> MAEQVKPAGVKPKGTVPPPKGNAPAPKANGAPGGASVIKEQDAAKMRRFLFQRTETRSTKWYQIFDTEKLDDEQVVGGHLALLGVLGFIMGIYYISGIQVFPWGAPGFHDNWFYLTIKPRMVSLGIDTYSTKTADLEAAGARLLGWAAFHFLVGSVLIFGGWRHWTHNLTNPFTGRCGNFRDFRFLGKFGDVVFNGTSAKSYKEALGPHAVYMSLLFLGWGIVMWAILGFAPIPDFQTINSETFMSFVFAVIFFALGIYWWNNPPNAAIHLNDDMKAAFSVHLTAIGYINIALGCIAFVAFQQPSFAPYYKELDKLVFYLYGEPFNRVSFNFVEQGGKVISGAKEFADFPAYAILPKSGEAFGMARVVTNLIVFNHIICGVLYVFAGVYHGGQYLLKIQLNGMYNQIKSIWITKGRDQEVQVKILGTVMALCFATMLSVYAVIVWNTICELNIFGTNITMSFYWLKPLPIFQWMFADPSINDWVMAHVITAGSLFSLIALVRIAFFAHTSPLWDDLGLKKNSYSFPCLGPVYGGTCGVSIQDQLWFAMLWGIKGLSAVCWYIDGAWIASMMYGVPAADAKAWDSIAHLHHHYTSGIFYYF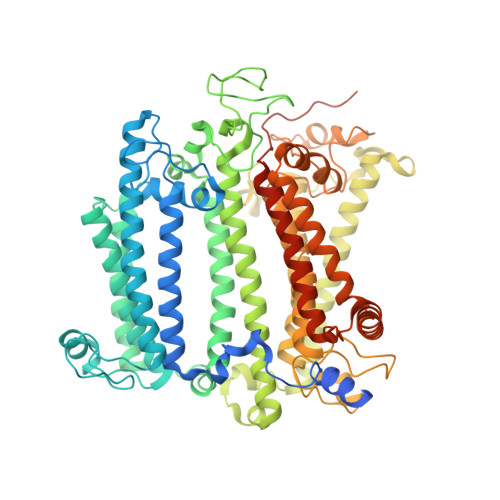WTETVTIFSSSHLSTILMIGHLVWFISFAVWFEDRGSRLEGADIQTRTIRWLGKKFLNRDVNFRFPVLTISDSKLAGTFLYFGGTFMLVFLFLANGFYQTNSPLPPPVSHAAVSGQQMLAQLVDTLMKMIA>[2x]VEYRNWSKPQCQITGFAPFSKDNSIRLSAGGDIWVTREPYVSCDPGKCYQFALGQGTTLDNKHSNGTVHDRIPHRTLLMNELGVPFHLGTRQVCIAWSSSSCHDGKAWLHVCITGD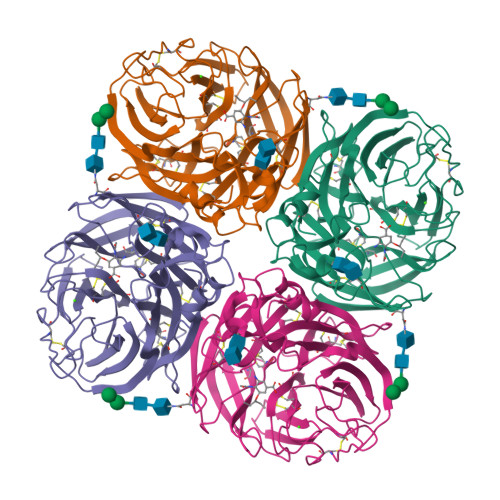DKNATASFIYDGRLVDSIGSWSQNILRTQESECVCINGTCTVVMTDGSASGRADTRILFIEEGKIVHISPLSGSAQHIEECSCYPRYPGVRCICRDNWKGSNRPVVDINMEDYSIDSSYVCSGLVGDTPRNDDSSSNSNCRNPNNERGTQGVKGWAFDNGNDLWMGRTISKESRSGYETFKVIGGWSTPNSKSQVNRQVIVDNNNWSGYSGIFSVEGKSCINRCFYVELIRGRPQETRVWWTSNSIVVFCGTSGTYGTGSWPDGANINFMPI>[4x]MATKPLIKPDVDLTDGNFYASRQAREAYRWMRANQPVFRDRNGLAAASTYQAVIDAE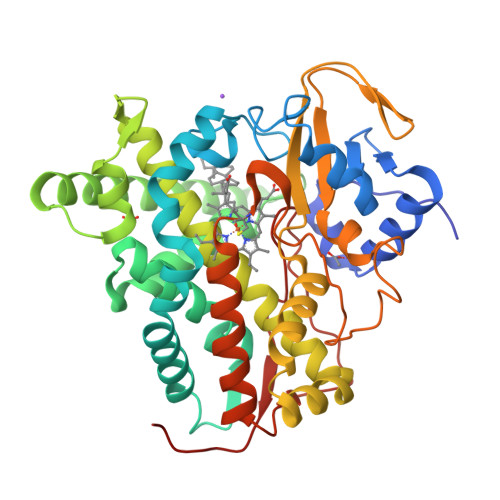RQPELFSNAGGIRPDQDALPMMIDMDDPAHLWRRKLVNAGFTRKRVKDKEHSIAQLCDTLIDAVCERGECDFVRDLAAPLPMAVIGDMLGVLPEQREMFLRWSDDLVTFLSSQVSQEDFQVTIDAFAAYNDFTRATIAARRAEPTDDLVSVLVSSEVDGERLSDDELVMETLLILIGGDETTRHTLSGGSEQLLRNRVQWDLLQSDRELLPGAIEEMLRWTAPVKNMCRMLTADTEFHGTALSKGEKIMLLFESANFDEAVFTDPEKFDIQRNPNSHLAFGFGTHFCMGNQLARLELSLMTARVVQRLPDLRLADQDSRLPLRPANFVSGLESMPVVFTPSRPLR>[4x]AAVILESIFLKRSQQKKKTSPLNFKKRLFLLTVHKLSYYEYDFERGRRGSKKGSIDVEK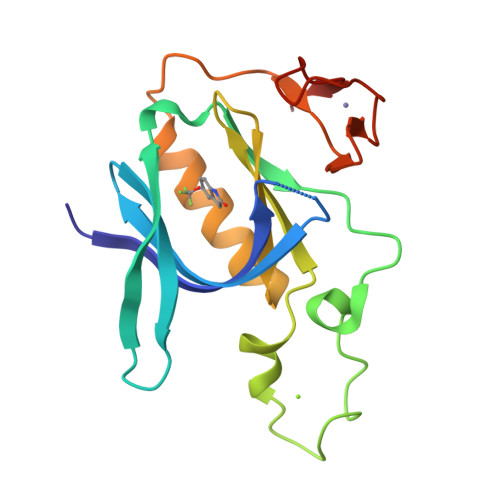ITCVETVVPEKNPPPERQIPRRGEESSEMEQISIIERFPYPFQVVYDEGPLYVFSPTEELRKRWIHQLKNVIRYNSDLVQKYHPCFWIDGQYLCCSQTAKNAMGCQILEN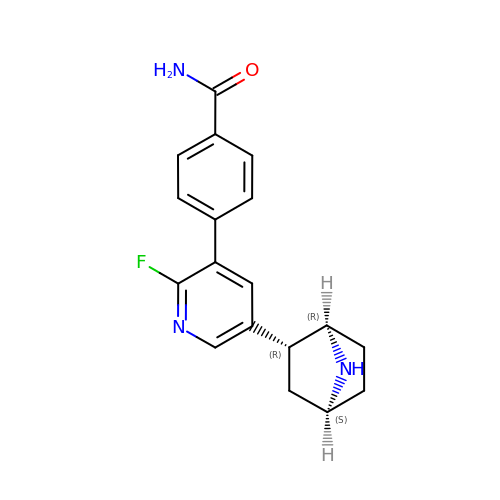4-[5-[(1~{R},2~{R},4~{S})-7-azabicyclo[2.2.1]heptan-2-yl]-2-fluoranyl-pyridin-3-yl]benzamide | C18 H18 F N3 O | QGEMISSKSNIODJ-SQWLQELKSA-N> MSISISYSTTYSGWTVADYLADWSAYFGDVNHAPGQVVDGSNTGGFNPGPFDGSQYALKSTASDAAFIAGGDLHYTLFSNPSHTLWGKLDSIALGDTLTGGASSGGYALDSQEVSFSNLGLDSPIAQGRDGTVHKVVYGLMSGDSSALQGQIDA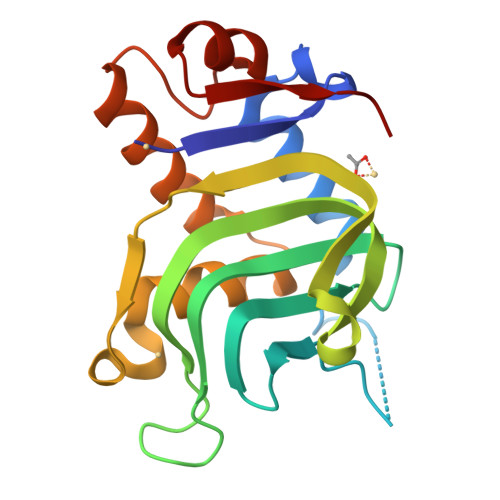LLKAVDPSLSINSTFDQLAAAGVAHATPAA> MSLEEQRTRDELKHKLLDLNQLHEQLAELRTICPSLLKLLHPETGTSRKFEKSAQEAIEKVNSFYTHLKSSQNVFDYAEKSLQADSSNLLPTYLYNSEDLSNDTENNETKSINGKSALDLKEPHHSELHDNDNFQNSDINIESFKGDIEASGSILTTHENKSFTLKLANELEFIFFHDTRGKFSVYCSSSKDDAITFSINRNNNFLGNLWSLMPKILDYQHLYSKPCDFCKSLISPVYLELPSVRRNANSTVKPTSKDILALHAECVPAQSDL;> METKWLLSKVPDDKSRFEIELEFVQMLSNPWYLNFLAQHKYFEDEAFLQYLEYMEYWREPEYVKFIIYPTCLHMLTLLKNPQFRNDISRADLSKQVNDEIYYEWLGKGLQQYGSADDATLSQPQQEEDEKKVDVKKENE;> MASGAPPSVDLTSIQWRMPEWVQSMGGLRTENVLEYFSQSPFYSHKSNNEMLKMQSQFNALDLGDLNSQLKRLTGIQFVIIHERPPFLWVIQKQNRLNENEVKPLTVYFVCNENIYMAPNAYTLLATRMLNATYCFQKALTKIEKFPQYNPQEGYTYPKLSNDNLEVDHSNTNEPADENKNQSIENADYSFSPEDFSVVRAFMQSLHSSKEAPDVK;> MEPNEGVQLFSAFPPPPPYYKLFTRENIEKVISNMEKEAKHEDDANTLQPKTEEEIESLAKLFKKPSCLTSGTYQMFGDTWRLDEAIPSLKEFGIPELYKDIKDGEDEIEVVEYDPKSNAIVGTSFTRVHDYDKNSPIENEKILEDDQHTAMKEKDNESDKTMKDVEEKTEPSLKKEEEDIQMKEPLDSQDTGAVSASSVNEGFRADQKSKDGETSDLIKIPRRAYELRFLSRSLMLNFLELLGIMAKAPEQFPSKVENIRVLLLNLHHLINDYRPHQSRESLIMLLEKQLKHEESQVELLRTHNRQMTETLEKYKSLDFNMEKEGDVIQQLKSSIKKPLSGAEDEQKSRSMFSKNDEKLKKSLELMEDVIKRDLS;> MEDISTEKTVESLEAIRHRIAQIVQSLTHFLAILHQSESLSPWPTIHKNFNILLSQIHSLSNNLAAHSHTLQTTSIYPSLEFPVKEQEPLLTTLLRTKALPEVEEWEANTLQEYEASISSQPKKKEANDAYQKDQLWDQARI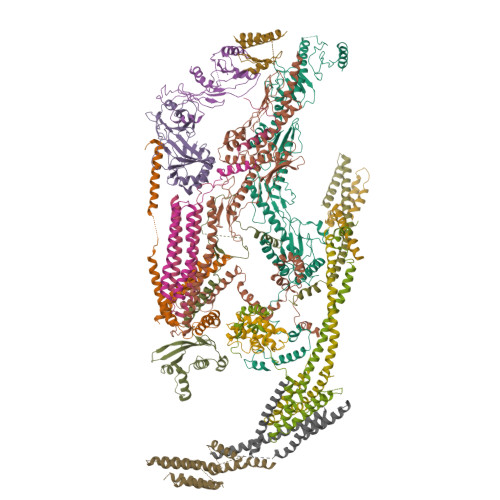IFMEERENYSWFDFVTRRQESEGEFVSQRQLEIDRATEEQNANQMLTDILSFMKSGKR;> MDPAHHIKDTSAELLSQQDFSILQSRLLEFLASQEARETVTASKELTLLRQGIRQLKEKVSKMEPEEMTVKEKKSIIEILKARIALKKAFLKMALSESNDTVVKKEDVRESPVDTFMENAT;> MTNSDDDLFSEKSTSSDTQQVQNILELEAKIPDILSSAGKCIEAIQLNNSLEDFRKYSKEFLETVEFISTGLRRQALELEKAEVPVVSLQPKKRYASTPLSNLIFDQSSKLIPKYC;> MEPPAIPHITEGFYPLPEIVETFSHHVLQELVSLAEVLPSMSNVEKKKKILDWLLRSRAFTMRLLVLARWVHLSPSVHRCIDVVAFLQGQKFCFQNLVHVLQDIRYQLSFARLRNSDLVTALDILSTGTSLRLANAPTSKLYMLSESPLSTKQILQTLHALNMLIRIRLSLYEIIPTPFQHFTIANGRCTFTVPNEFSVSLTTNSQDPKSTGISFQWIVVDFQFHLPDFSSTPAKYRVFIELHLNEEIAAAFVLQKPILPLIYNILHKFCLYQRLNLLSQQTFQLSRESWLGHLRGVYDEKPPRLRLYYWPQLNVKKEGKPGKIGHYIHIFVNTQPISAFERTLSSKRSSCEYDHFLLLVEWHHDGIVEHVPLDDHMDAQHLLLLITQKHAQLILEQIRKELHPNIFSEHVGGGLKIHVFDNEIIVKVNSVTGRLVLSSSASPLSPPRHLRAAEKNIALNTQPPAQILNRLYFFCIQTQLLEVAQCAELHAVQGYYSFPYLTFSKGKWRKDGDSLWVLAYNVESNSWSVRLLNAAGQTLYTQDVHTTKGTLSIESFSRLSYLLEVQILLFNVQTACQARGMPFEYLPIPPKALIEDDFTTYVQTGCLCIMMPSSNEDMLPVVFVRAHDGQLIFDSRIKGKLPYQSETETEKNCYIDWRTGRITIRVQNFSSFEKTWIGLLKLVALSKTSAFNVDCITLKHVDFTYLDDEKFRATIHDDNTFTLHFFNRHSPFHLISQFLQDTFSDGPSAIQPLRVIMDRTRGVLVAQELGYVVLARSLRQYRIILSKNHGIQVLLNRHGCILQDLSYLSADSRYLEGTQTLTSQWEPCSWLNTVWEGDLGDDELNGQIEAAPEMHLIKMNKTADLTAILKRILAISRKKXXXXXXXXXXXXXXXXXXXXXXXXXXXXXXXXXXXXXXXXXXXXXXXXXXXX;> MAEEANKDADISSLSLSLDPEIIGGQNNFLENNLQQIFQKIIQERGPFRDLKEEDLQKELQKESIKDESSAKSSETENVLEFATLDSKRNVNDTEVESMDSQAYKKELIEQIMIAQTECSLALDMTSLLLSKFKENSIETISPFLKSTVPPSSLQFSRSQPPESKESDATLAKCWKEKSLTSSCKFLFEAKERLTSVVETEHEYYTELVKVKEASWPLFNSQGSNHLSVQYSCLGGISLGLGLIRMKPESKSFEVQSSLLYSQAALKISILNKDRDEIGSSTWSWPSQNCNSVLLKDIYKLQEILFEMDIWNSLLQEAQSCGNQGVNFTGDEILVPISDDHVVRITLETSSKNTESGFTEDKKSNEDTSTNFVTIKQEKELLKCLCDTLNAIAHILFLKHCRKSDRRSQQPELYMAIDANAPLILRPLIFYYNLNQESLEFQRWLKQRDISFKFMPNYPWEKAKDFLELENSLSINRLSISWRIMVSNFEPAIFIQHTPTLHGTDKSVWRCKDQYSSNQFSSLKNVCQYIEHHINSLSRRSKKTE;> MQELYLLGVVPSRRFEAVVNSLSKTLDGPKTILEFWVVYRPKDVPPNLPRQPDSWLRLCSNIESHDETDTEWSKNTQWSMYLEGNSEPKREDKCGIRPVNRAKLTNGSVTEFVEKMGYEFSHEYIIQGLEYFFFDTTVRIYQTLIPSQQRSIKPPFHPMNEEQPWILHVYTHVADASNQVAMAKAEANLTKVKTLLSAFCDLKNVRL;> MPVHGVIYYSSPSMATFLSPAQDNLVRTYFAQHLKKWVVQYKLYRNAVTPKTLEFLKQNINPSMLACVDEATMIDAEPELEDIIVRTKLWNFRQSFTIEGSIYEVGSFKVAIANVLQKSVWKGILFHVTYDGTESVDLARPIIQEFFLKCFLQNNKSVTPVYESFFNQPRHSLDSKLLLQLFKQRIDTVSQRT;> MACRCTQLQDTIDEVATQFYSSIHYLSSHHDFVPLPGQEKVSDSKVNPISAEELQFAQRDLAKDLVTKFMQIDTLINQLPGISTAPKHQLEKIKKLQNSIEEKQLERKSLESENEDLKLQLAKRIETFGRLSCVLFQP;> MSSDSFQRQLVQRTNTLNSSIDNATLTILSRFQDILDIAINEGKDKYTVAPEVYQIECHTVSMVRAVEQLLDVSRQIKSYWLTNSLSTSFPTVDYSEPDLEKVKRTLTKLQNHLLEVSLIEPEASETTEAPTVSDT> YIATR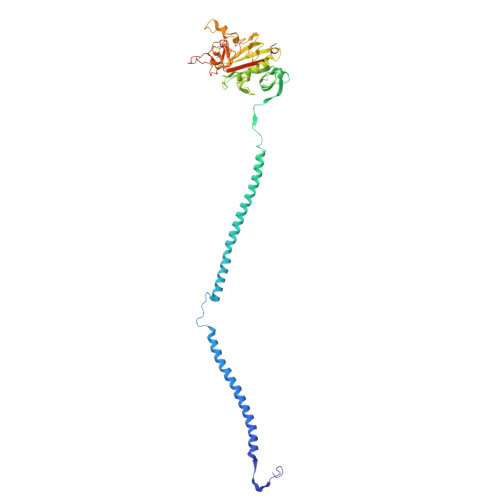ENCCILDERFGSYCPTTCGIADFFNKYRLTTDGELLEIEGLLQQATNSTGSIEYLIQHIKTIYPSEKQTLPQSIEQLTQKSKKIIEEIIRYENTILAHENTIQQLTDMHIMNSNKITQLKQKIAQLESHCQEPCKDTAEIQETTGRDCQDIANKGARKSGLYFIKPQKAKQSFLVYCEIDTYGNGWTVLQRRLDGSEDFRRNWVQYKEGFGHLSPDDTTEFWLGNEKIHLITTQSTLPYALRIELEDWSGKKGTADYAVFKVGTEEDKYRLTYAYFIGGEAGDAFDGFNFGDDPSDKSYTYHNGMRFSTFDNDNDNFEGNCAEQDGSGWWMNRCHAGHLNGPYYIGGVYSRDTGTNSYDNGIIWATWRDRWYSMKKTTMKIIPFNRLSIDGQQHSGGLKQVGDS> GSMVEATAQETDRPRFSFSIAAREGKARTGTIEMKRGVIRTPAFMPVGTAATVKALKPETVRATGADIILGNTYHLMLRPGAERIAKLGGLHSFMGWDRPILTDSGGYQVMSLSSLTKQSEEGVTFKSHLDGSRHMLSPERSIEIQH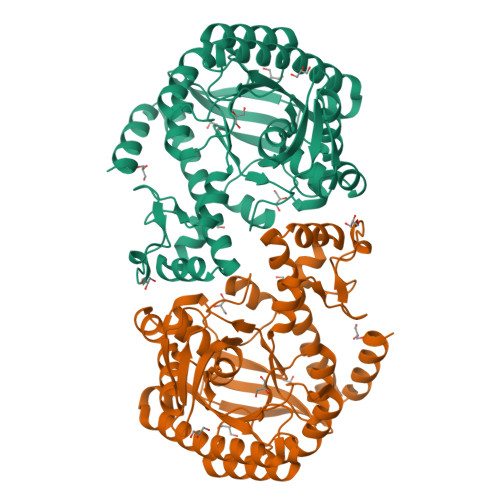LLGSDIVMAFDECTPYPATPSRAASSMERSMRWAKRSRDAFDSRKEQAENAALFGIQQGSVFENLRQQSADALAEIGFDGYAVGGLAVGEGQDEMFRVLDFSVPMLPDDKPHYLMGTGKPDDIVGAVERGIDMFDCVLPTRSGRNGQAFTWDGPINIRNARFSEDLKPLDSECHCAVCQKWSRAYIHHLIRAGEILGAMLMTEHNIAFYQQLMQKIRDSISEGRFSQFAQDFRARYFARNS>MRGSHHHHHHGSAEKQERVQHLHDIRDLHRYYSSESFEYSNVSGKVENYNGSNVVRFNPKDQNHQLFLLGKDKEQYKEGLQGQNVFVVQELIDPNGRLSTVGGVTKKNNKTSETNTPLFVNKVNGEDLDASIDSFLIQKEEISLKELDFKIRQQLVNNYGLYKGTSKYGKIIINLKDENKVEIDLGDKL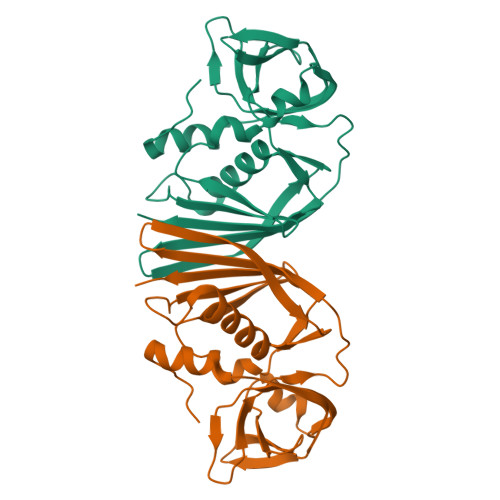QFERMGDVLNSKDIRGISVTINQI[2x]>[6x]HPETLVKVKDAEDQLGARVGYIELDLNSGKILESFRPEERFPMMSTFKVLLCGAVLSRIDAGQEQLGRRIHYSQNDLVEYSPVTEKHLTDGMTVRELCSAAITMSDNTAANLLLTTIGGPKELTAFLHNMGDHVTRLDRWEPELNEAIPNDERDTTMPVAMATTLRKLLTGELLTLASRQQLIDWMEADKVAGPLLRSALPAGWFIADKSGAGERGSRGIIAALGPDGKPSRIVVIY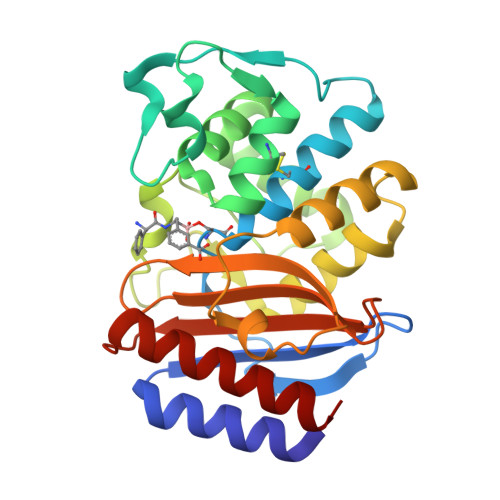TTGSQATMDERNRQIAEIGASLIKHW> MMIVQRVVLNSRPGKNGNPVAENFRMEEVYLPDNINEGQVQVRTLYLSVDPYMRCRMNEDTGTDYITPWQLSQVVDGGGIGIIEESKHTNLTKGDFVTSFYWPWQTKVILDGNSLEKVDPQLVDGHLSYFLGAIGMPGLTSLIGIQEKGHITAGSNKTMVVSGAAGACGSVAGQIGHFLGCSRVVGICGTHEKCILLTSELGFDAAINYKKDNVAEQLRESCPAGVDVYFDNVGGNISDTVISQMNENSHIILCGQISQYNKDVPYPPPLSPAIEAIQKERNITRERFLVLNYKDKFEPGILQLSQWFKEGKLKIKETVINGLENMGAAFQSMMTGGNIGKQIVCISEEIAENLY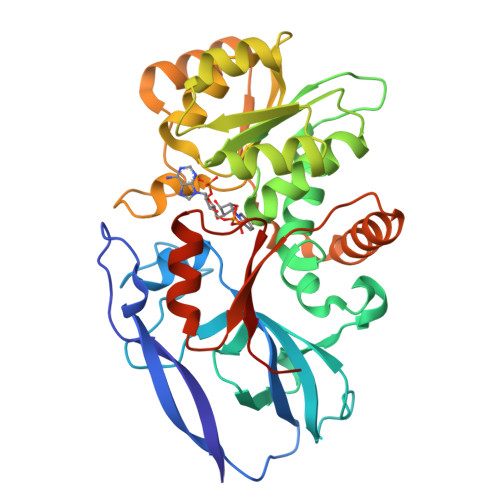FQ>GSGPPGPPGPPGPPGARGQAGVMGFPGPPGPPGPPGRAPTDQHIKQVCMRVIQEHFAEMAASLKRPDSGAT[2x];>[2x]GSGPPGPPGPPGPPGARGQAGVMGFPGPPGPPGPPGRDATDQHIVDVALKMLQEQLAEVAVSAKREALGAV;>GSGPPGPPGPPGPPGARGQAGVMGFPGPPGPPGPPG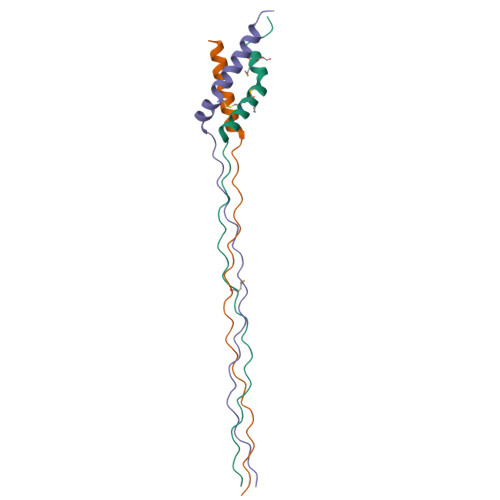KEASEQRIRELCGGMISEQIAQLAAHLRKPLAPGSI[2x]> HRPEGLEQLEAQTNFTKRELQVLYRGFKNECPSGVVNEETFKQIYAQFFPHGDASTYAHYLFNAFDTTQTGSVKFEDFVTALSILLRGTVHEKLRWTFNLYDINKDG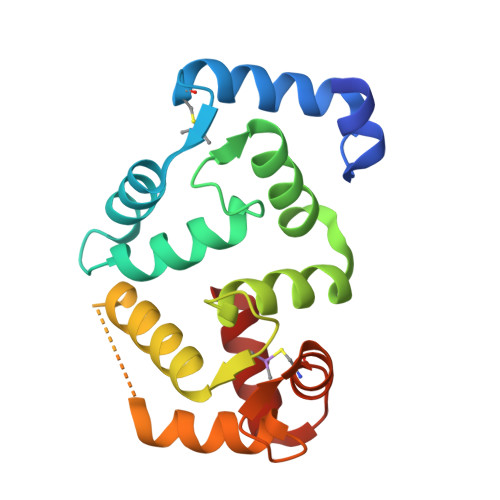YINKEEMMDIVKAIYDMMGKYTYPVLKEDTPRQHVDVFFQKMDKNKDGIVTLDEFLESCQEDDNIMRSLQLFQNVM>[3x]PPGPPGP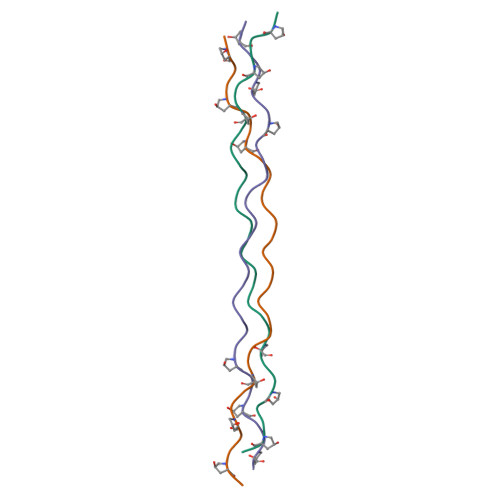PGKPGANGLSGERGPPGPPGPPG>GSHMGDLKYSLERLREILERLEENPSEKQIVEAIRAIVENNAQIVEAIRAIVENNAQIVENNRAIIEALEAIGGHNKILEEMKKQLKDLKRSLERG[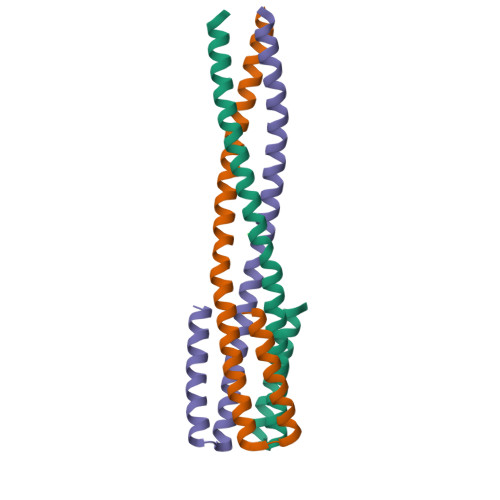3x]>MKKVALITGITGQDGAYLAELLLQKGYAVHGIKRRTSQFNTARIDHLYHDPHEQGVDLTLHHGDLTDTSSLVRIMQLVRPDEVYNLGAQSHVAVSFEEPEYTANSDALGALRLLEAIRILGMEKQTRYYQASTSELYGLVQEIPQKETTPFYPRSPYAAAKLYAYWITVNYREAYGIYACNGILFNHESPLRGETFVTRKITRALARIKIGNQNRLYLGNLDSLRDWGHARDYVEMQWLMLQQDQPEDFVIATGKQYS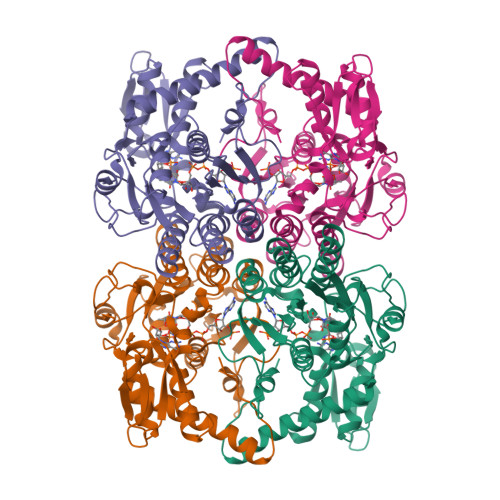VREFVTLAAKDIGIEMRWEGSGEAEKGYDAKTGACIVEVDPRYFRPAEVETLLGDATKAHQKLGWKPKISFETLVSEMIAEDLAAAARENLLREHGHQFFAPKEGHHHHHH[4x]> KIPEHLIGKGAEADIKRDSYLDFDVIIKERVKKGYRDERLDENIRKSRTAREARYLALVKDFGIPAPYIFDVDLDNKRIMMSYINGKLAKDVIEDNLDIAYKIGEIVGKLHKNDVIHNDLTTSNFIFDKDLYIIDFGLGKISNLDRDKAVDLIVFKKAVLSTHHEKFDEIWERFLEGYKSVYDRWEIILELMKDVERRARYVE;> MDPMIIRGIRGARINNEIFNLGLKFQILNADVVATKKHVLHAINQAKTKKPIAKSFWMEILVRASGQRQIHEAIKIIGAKDGNVCLICEDEETFRKIYELIGGEIDDSVLEINEDKERLIREIFKIRGFGNVVERVLEKIALIELKKE;> PMICLGLEGTAEKTGVGIVTSDGEVLFNKTIMYKPPKQGINPREAADHHAETFPKLIKEAFEVVDKNEIDLIAFSQGPGLGPSLRVTATVARTLSLTLKKPIIGVNHCIAHIEIGKLTTEAEDPLTLYVSGGNTQVIAYVSKKYRVFGETLDIA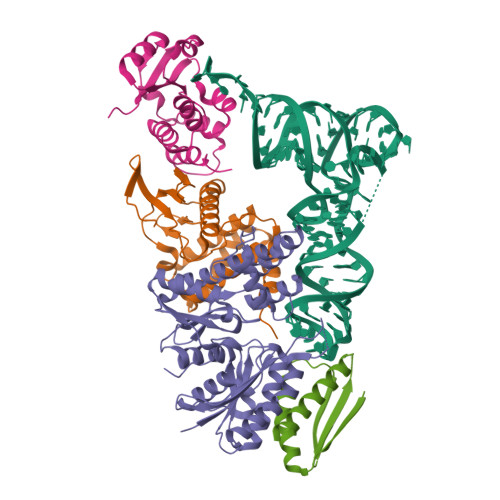VGNCLDQFARYVNLPHPGGPYIEELARKGKKLVDLPYTVKGMDIAFSGLLTAAMRAYDAGERLEDICYSLQEYAFSMLTEITERALAHTNKGEVMLVGGVAANNRLREMLKAMCEGQNVDFYVPPKEFCGDNGAMIAWLGLLMHKNGRWMSLDETKIIPNYRTDMVEVNWI;> MKAKRVQAKIEIEFPSEDVAKVVYEAVLYEHLSVPYRRSEIDFKLEGKKIILDIKATDSSALRGTVNSYLRWIKAAIDVIEVGSGSGSGSGSGMKAKRVQAKIEIEFPSEDVAKVVYEAVLYEHLSVPYRRSEIDFKLEGKKIILDIKATDSSALRGTVNSYLRWIKYAIDRIEV> GPHMRTFFVGGNWKANPKTVEEAEKLIEMLNGAKVEGNVEVVVAAPFIFLPTLQQKLRKDWKVSAENVFTKPNGAFTGEVTVPMIKSFGIEWTILGHSERRDILKEDDEFLAAKAKFALENGMKIIYCCGEHLSEREAGKASEFVSAQIEKMIPAIPAGKWDDVVIAYEPIWAIGTGKVASTQDAQEMCKVIRDILAAKVGADI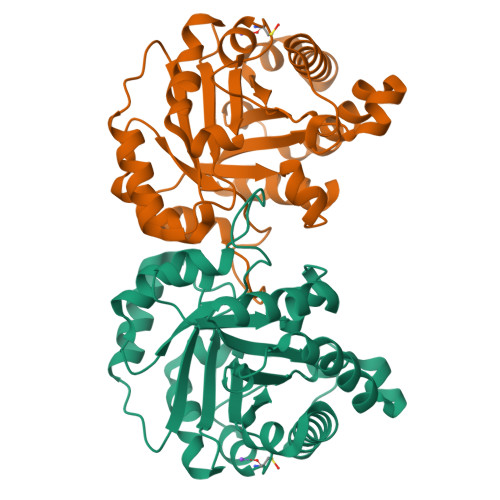ANKVRILYGGSVKPNNCNELAACPDVDGFLVGGASLEPGFINIVNSNVHSK> SMPRDNMASLIQRIARQASLTFRGSGGGRGASDRDAASGPEAPMQPGFPENLSKLKSLLTQLRAEDLNIAPRKATLQPLPPNLPPVTYMHIYETDGFSLGVFLLKSGTSIPLHDHPGMHGMLKVLYGTVRISCMDKLDAGGGQRPRALPPEQQFEPPLQPREREAVRPGVLRSRAEYTEASGPCILTPHRDNLHQIDAVEGPAAFLDILAPPYDPDDGRDCHYYRVLEPVRPKEASSSASDLPREVWLLETPQADDFWCEGEPYPGPKVFP;> XYIVKTFWKGSHRQCX

N-terminal cysteine oxidases (NCOs) act as enzymatic oxygen (O2) sensors, coordinating cellular changes to hypoxia in animals and plants. They regulate the O2-dependent stability of proteins bearing an N-terminal cysteine residue through the N-degron pathway. In animals, the Cys branch of the N-degron pathway is regulated by the NCO 2-aminoethanethiol dioxygenase (ADO), which also plays a role in cysteamine catabolism and taurine biosynthesis. Biochemically, ADO is a non-haem iron-dependent thiol dioxygenase (TDO) from the cupin fold family of enzymes, consisting of a conserved double stranded β-helix (DSBH) core in which the active site is situated.

To overcome these issues, CP6 was used as a molecular scaffold to graft substrate moieties, anticipating that its binding and inhibition properties would enhance substrate complex formation by increasing association and reducing turnover. CP6-L8 protrudes into the active site of ADO without contributing to binding, rendering it a viable site for substrate moiety installation. In the first instance, CP6-L8 was replaced with ornithine (Orn; O) or lysine (Lys), allowing the sidechain amine to be coupled to Cys or serine (Ser), the latter of which is an amenable substrate analogue. This generated a pseudo-N-terminus with conformational and rotational flexibility, which could reach the ADO active site metal (a distance of 7.5 Å). The association of these CP6-substituents was assessed by SPR using SCK, revealing that Cys and Ser conjugated to a Lys sidechain enhanced binding relative to unmodified CP6. The Ser residue of CP6-L8K-Ser coordinates the metal centre in a bidentate arrangement through ligation of both the hydroxyl and amine group, leaving one water molecule trans to ADO-H112, which is the putative site of oxygen binding and activation. The water molecule trans to ADO-H112 also forms a hydrogen bond with ADO-D206, which points towards the metal centre through an additional interaction with the amine of CP6-L8K-Ser. The crystal structures of cobalt-incorporated ADO in complex with CP6-L8K-Ser and CP6-L8d-Gly-Ser provide valuable information on substrate analogue binding. However, they do not reflect native conditions in which an iron cofactor interacts with an Nt-Cys residue.1,5-dimethyl-3~{H}-indol-2-one | C10 H11 N O | 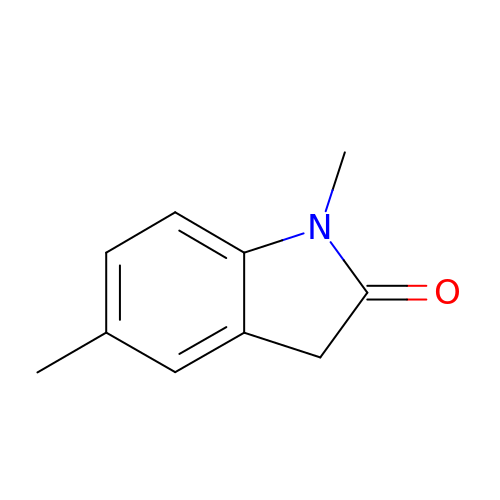OSKUFVWHNUVFJR-UHFFFAOYSA-N The first dedicated enzyme of the MEP pathway, deoxyxylulose phosphate reductoisomerase (DXR; E.C. 1.1.1.267), is rate-limiting for MEP pathway activity. In contrast, nonprimate-associated staphylococcal species, including S. pseudintermedius and S. schleiferi, utilize the MEP pathway for isoprenoid biosynthesis. S. schleiferi DXR is a physiologic dimer with each monomer related by crystallographic symmetry. The monomer consists of three regions: an N-terminal α/β-domain with a central 7-stranded β-sheet (β1-β7) and 7 α-helices that serves as the nucleotide binding site; a middle region of the protein that includes a second β-sheet (β8-β11) and 4 α-helices (α8 and α12-α14); and a C-terminal α-helical domain (α9-α11 and α15-α18) that locks FSM into the active site.

To establish the structural basis of FSM action, we solved the three-dimensional structures of S. schleiferi DXR as an apoenzyme and a FSM complex to 2.15 Å and 2.89 Å resolution, respectively. Comparison of the S. schleiferi DXR apoenzyme and FSM complex structures reveals how the C-terminal capping region (α9-α11 and α16–18) shifts position to allow for the α10-α11 loop to position Trp196 adjacent to the inhibitor. A DALI search identified multiple DXR from Escherichia coli, Plasmodium falciparum, M. tuberculosis, and other microbes (Z-scores: 49–51; r.m.s.d. ~1.6 Å2 for 370–400 Cα-atoms; 39–40% amino acid sequence identity)[31–36]. Of note, the staphylococcal DXR enzyme appears somewhat distinct from previously characterized orthologs, particularly in the α10-α11 loop sequence, which could be explored with additional SAR studies.

>MKNIAILGASGSIGQQAIDVIARHPESFNLISFTVGKNIEFAIEVIEKFKPEIVSVQDEADVERLKPYHSNIVSGRQGLIDVSTYEKNDLVLNALLGSVGLEPTMKAIEAGKNIALANKETLVVAGKLVMTHAKRYGVDILPVDSEHAAIFQCLNGEDMHKIKNVTITASGGSFRELTREQLEHVTVGDALNHPNWSMGNKITIDSATMMNKGFEVIEAKWLFDLKIDQIKTILHKESIIHSLVEFVDTSVMAQLGTPDMRMPIQYAFTYPERIEHRAPSLDLVQVAQLHFQEMDLDRYRCLKFAYDALRIGGSMPVVLNAVNEVAVAKFLNHEITFLEIEHMIEREMSAHEVIPDPSLEEILEIDHYYKTKSYEV[2x]>MSKLDLGRVDLLSMLGNSSSAGVDTAKGVIPFSTSGATWAVPRLSEDGITSHFLRRRGYVTMTQGGSRDQNAAVRKILSLIIAYDIQTQACFFISNEESMRITMAETMGVKDRPNARTNSWAEVSDSDINRGIAKALKEGNLTLDENQKDGFMKLVHAFVADILAQSGHYKPVTSVTYFSAPIDMESDYLDPFSIAIIRDVLDDSPFSELRYDARAMSELEDRDVPITRFSRVMAQMGNAMVRNIMVLNEAAQRKLRGLAVVGEIVHGRVRAPVRYLNDSFIQTLRSNINFHLLTRTTPERWAQSWIQAFGSLKGWVDAINGIADATTEEEKKKLAMQTSMDLELLSDLTPLIRDAATSVEKFVTFAP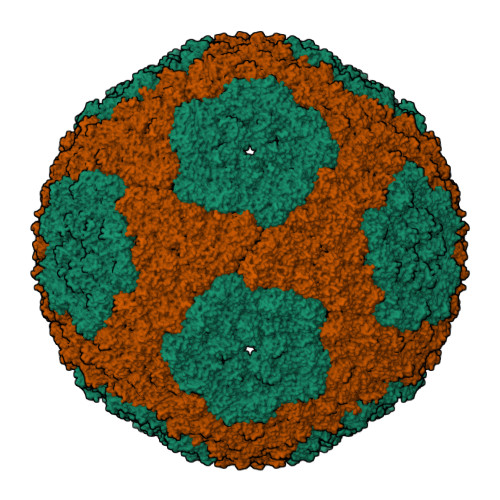LSFYQGLGSVTQIRALDSSTNLAAVIVRYAAKEINLIPAYQSFQVPTVDVGVKKTAIMDQRLSLQLPEFSEDQFFGMLEQRMQNMSDSEVAELVDRIAKGETPFGDVVKQLPGTSTLLVTNGYYMGGLLTNEDKIIPGDASVPALLYMQAASFASSVRFPPGEYPVFHHESSNGDVRLTDQVSADAQLSHSAVETANPLNFLVACNVSVHTPSIAIDIIEPMPDLTRRGTTEYVHKGEIKVAAIPSLPPKSADRKAQVSRETAKFERVLYKARKGGAQVAAPIDLESLFGIAVNLAVPTVKHVYSPDSKTKLALDIIKGLESDGDKAAATRLLMTLARAYTGTYSSLGLRRRDEITGIAAQPSDVAMQEFALQSGVQTLKAVAKHTGIMEVATIEMVEEKVRSLDDNRFYEIAAEVVLRALKGM[2x]>[4x]PQFEKIEGRMIR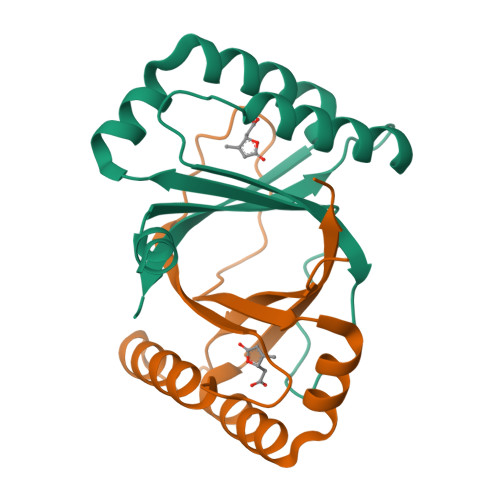ILYLLVKPESMSHEQFRKECVVHFQMSAGMPGLHKYEVRLVAGNPTDTHVPYLDVGRIDAIGECWFASEEQYQVYMESDIRKAWFEHGKYFIGQLKPFVTEELV>GYSSEKIPVTGSGFVAKDDSLRTFFDAMALQLKEPVIVSKMAARKKITGNFEFHDPNALLEKLSLQLGLIWYFDGQAIYIYDASEMRNAVVSLRNVSLNEFNNFLKRSGLYNKNYPLRGDNRKGTFYVSGPPVYVDMVVNAATMMDKQNDGIELGRQ[15x]

The bacterial injectisome, or type III secretion system (T3SS), is a specialized syringe-shaped protein-export system utilized by many pathogenic Gram-negative bacteria for the injection of virulence proteins (effectors) into host cells. The injectisome can be divided into three major regions: the inner- (IM) and outer-membrane (OM) spanning basal body with associated export apparatus and ATPase components, an extracellular needle, and a terminating pore inserted into the host cell membrane called the translocon. The major structural scaffold of the basal body is comprised largely of three proteins that arrange into a series of highly oligomerized, concentric rings: two intimately associated proteins localized to the IM - PrgK/EscJ/MxiJ and PrgH/EscD/MxiG, and a third protein belonging to the secretin family of OM proteins, InvG/EscC/MxiD (Salmonella enterica serovar Typhimurium SPI-1, Enteropathogenic Escherichia coli (EPEC) LEE and Shigella dysenteriae nomenclature, respectively). In summary, we report the crystal structures for the cytoplasmic and periplasmic domains of PrgH and InvG, two of the main basal body components of the prototypical Salmonella SPI-1 injectisome.

The stoichiometry of the T3SS OM secretin has been a matter of debate, with numbers between 12 and 14 proposed and recent studies favouring 12 for the secretins of other systems. Unexpectedly, the recent EM analysis of the SPI-1 basal body suggested a stoichiometry of 15. We therefore generated ring models with stoichiometries of 12, 14 and 15. Based on the docking results, the 12-mer model appears incompatible with the target region of the EM maps, having significantly lower interface energies and worse map correlation. Use of the higher resolution map, however, clearly favours the 15-mer assembly, with the 14-mer configuration having significantly worse correlation to the EM map and Rosetta energy. Using the high-resolution map, the modelling converged on two opposite modes – a “helix in” conformation and a “helix out” conformation” referring to the orientation of the helix in the N1 domain of InvG. The “helix in” mode shows excellent agreement with our previous biotinylation and cross-linking experiments, and better fit with the EM map. Finally, for InvG we observed a loop (residues 95–99) forming a series of side-chain contacts with the adjacent subunit. Mutation of Gln97 within the loop (which forms a hydrogen bond with the adjacent molecule) to leucine – but not alanine - abrogates secretion (top). Furthermore, we observed a positively charged interior collar of the InvG ring corresponding to the N0 domain, where residues are proposed to be in contact with the inner rod and socket.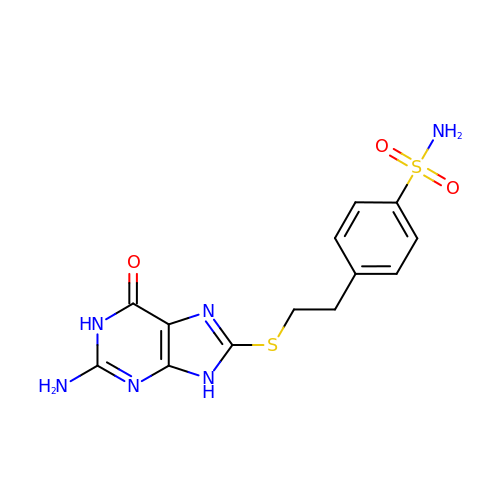4-{2-[(2-amino-6-oxo-6,9-dihydro-1H-purin-8-yl)sulfanyl]ethyl}benzene-1-sulfonamide | C13 H14 N6 O3 S2 | CQRWHGAPSZBUKT-UHFFFAOYSA-N2-(2-aminopyridin-1-ium-1-yl)ethanol | C7 H11 N2 O | 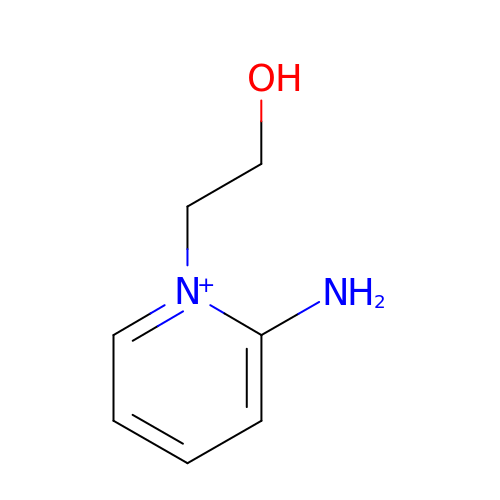BFRGFNNQJWMZSX-UHFFFAOYSA-N>MEALKRKIEEEGVVLSDQVLKVDSFLNHQIDPLLMQRIGDEFASRFAKDGITKIVTIESSGIAPAVMTGLKLGVPVVFARKHKSLTLTDNLLTASVYSFTKQTESQIAVSGTHLSDQDHVLIIDDFLANGQAAHGLVSIVKQAGASIAGIGIVIEKSFQPGRDELVKLGYRVESLARIQSLEE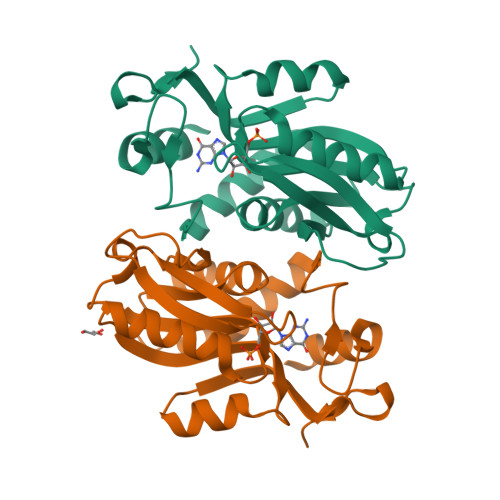GKVSFVQEVHS[2x]> 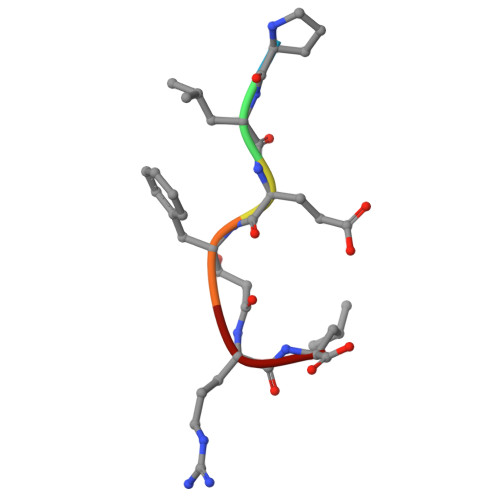PLEFRL>SEELEKALSKLSEREAMVLKMRKGLIDGREHTLEEVGAYFGVTR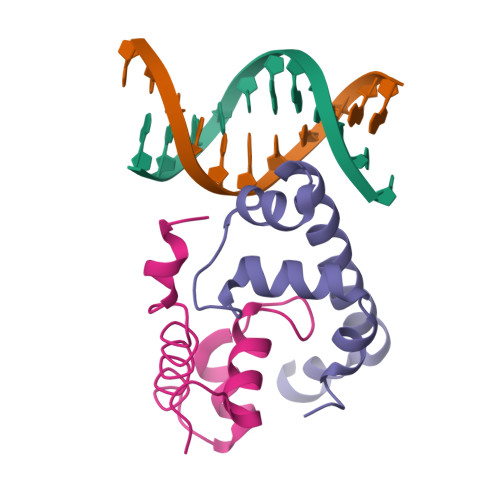ERIRQIENKALRKLKYHESRTRKLRDFLE[2x]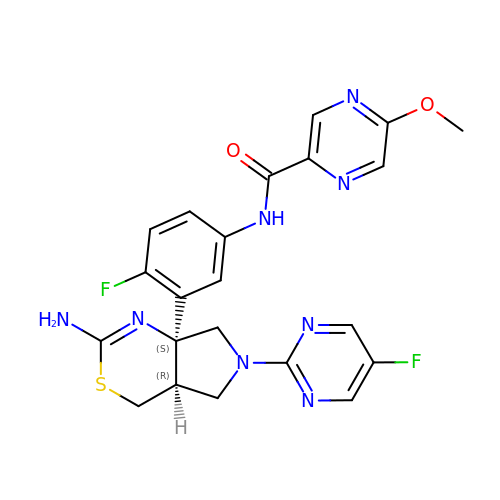N-{3-[(4aR,7aS)-2-amino-6-(5-fluoropyrimidin-2-yl)-4a,5,6,7-tetrahydropyrrolo[3,4-d][1,3]thiazin-7a(4H)-yl]-4-fluorophenyl}-5-methoxypyrazine-2-carboxamide | C22 H20 F2 N8 O2 S | VQSRKMNBWMHJKY-YTEVENLXSA-N> MIERLNSPFLRAAALFTIVAFSSLISTAALAENNPSDTAKKFKVVTTFTIIQDIAQNIAGDVAVVESITKPGAEIHDYQPTPRDIVKAQSADLILWNGMNLERWFEKFFESIKDVPSAVVTAGITPLPIREGPYSGIANPHAWMSPSNALIYIENIRKALVEHDPAHAETYNRNAQAYA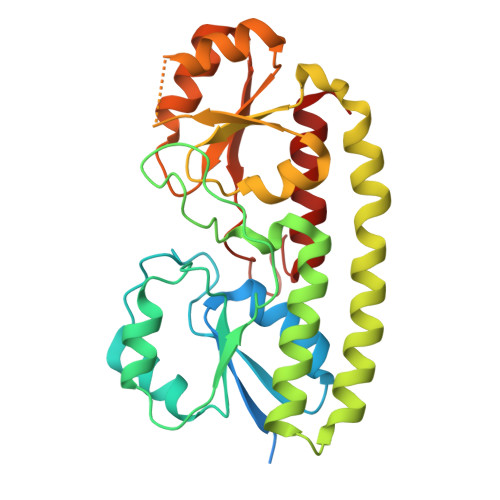EKIKALDAPLRERLSRIPAEQRWLVTSEGAFSYLAKDYGFKEVYLWPINAEQQGIPQQVRHVIDIIRENKIPVVFSESTISDKPAKQVSKETGAQYGGVLYVDSLSGEKGPVPTYISLINMTVDTIAKGFGQ> GEEQMRLPSADVYRFAEPDSEENIIFEENMQPKAGIPIIKAGTVIKLIERLTYHMYADPNFVRTFLTTYRSFCKPQELLSLIIERFEIPEPEPTEADRIAIENGDQPLSAELKRFRKEYIQPVQLR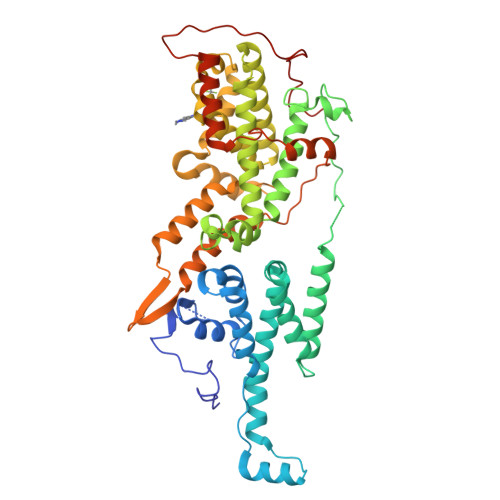VLNVCRHWVEHHFYDFERDAYLLQRMEEFIGTVRGKAMKKWVESITKIIQRKKIARDNGPGHNITFQSSPPTVEWHISRPGHIETFDLLTLHPIEIARQLTLLESDLYRAVQPSELVGSVWTKEDKEINSPNLLKMIRHTTNLTLWFEKCIVETENLEERVAVVSRIIEILQVFQELNNFNGVLEVVSAMNSSPVYRLDHTFEQIPSRQKKILEEAHELSEDHYKKYLAKLRSINPPCVPFFGIYLTNILKTEEGNPEVLKRHGKELINFSKRRKVAEITGEIQQYQNQPYCLRVESDIKRFFENLNPMGNSMEKEFTDYLFNKSLEIEPRNPKPLPRFPKKYSYPLKSPGVRPSNPRPGT> PVWGCASTRGRS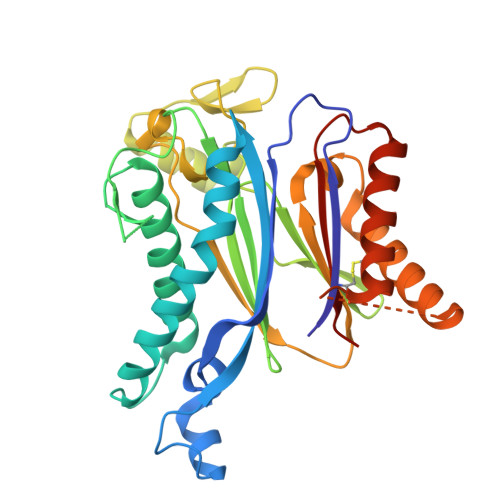AEMEDASAAVPRFADVPVRLLASRRDLDALGLDADALRLPAHLFGVFDGHGGAEVANYCRERIHVVLSAALARLGKNLGEMGEVDMKEHWDDVFTKCFQRVDDEVSGRVTRVVNGGGEVRSEPVTAENVGSTAVVALVCSSHVVVANCGDSRIVLCRGKEPVALSIDHKPDRKDERARIEAQGGKVIQWNGYRVSGILAMSRSIGDRYLKPFVIPKPEVMVVPRAKDDDCLILASDGLWDVVSNEEACKVARRQILLWHKNNGAASPLSDEGEGSTDPAAQAAADYLMRLALKKGSEDNITVIVVDLKPRKKLKN> MPVITVNTNVAEKSIPVFFQAALTNMMTKALQKPKEVMFVDLRSGANIMMGGDRNPCVFATVECIGRLNPTSNLAMARDMEDMFIEHLNVRRERIVIRFIP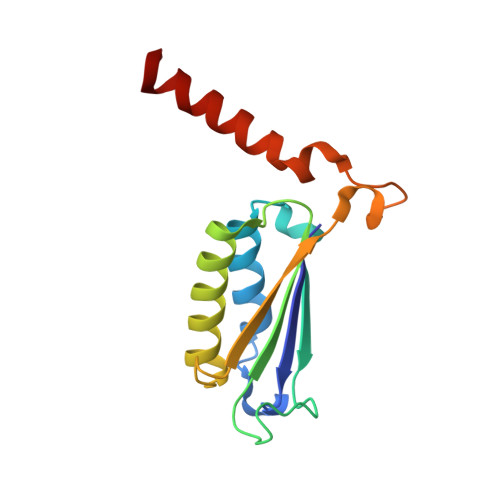VPALFCSFNGALHDVSIERDEDIISQAIAEYLHHHHH Beta-glucosidases (β-glucosidases) are key cellulolytic enzymes that catalyze the hydrolysis of cellobiose to glucose. They are terminal enzymes of the cellulase system as they act during the final step of the cellulose degradation. Beta-glucosidases (β-glucoside glucohydrolases, EC 3.2.1.21; BGL) have been found in the glycoside hydrolase (GH) families GH1, GH3, GH5, GH9, GH30, and GH116 of the CAZy database. They are anomeric configuration-retaining enzymes that operate through the canonical double-displacement glycosidase mechanism, except those of the GH9 family. Here, we report the crystal structure of a β-glucosidase from the thermophilic filamentous fungus Chaetomium thermophilum (CtBGL) at a resolution of 2.99 Å, and compare it with other β-glucosidases of the GH3 family.

The structure of CtBGL consists of three distinct domains, similar to other GH3 family members: A catalytic triose phosphate isomerase (TIM) barrel-like domain (Leu51–Ser354), an α/β sandwich domain (His396–Gly596) and a FnIII (fibronectin type III) domain (Thr663–Gln867) with a prominent insertion region (677–766). A linker region (residues 355–394) connects domain 1 to domain 2 and a second linker region (600–662) connects domain 2 to domain 3. The active site is located in a shallow pocket near the interface of the first and second domain. A molecule of β-d-glucose (BGC) was fitted at the active site based on residual electron density observed in electron density Fo–Fc difference maps. The source of the β-d-glucose is most likely the growth medium used as no β-d-glucose was used during crystallizations or soaking. Two catalytic residues were identified, Asp287 (nucleophile) at the N-terminal TIM-barrel domain and Glu517 (acid/base) at the sandwich α/β domain II. Potential glycosylation sites were observed in the CtBGL structure in 10 positions, all in Asn residues. A total of 27 glycan moieties were found in CtBGL. The N-glycan at CtBGL Asn329 was located in domain I of the enzyme and consisted of eight monosaccharides (two GlcNAc, five α-d-Man, and one β-d-Man). CtBGL has been found to be thermostable at 50 °C and to retain half of its activity after incubation at 65 °C for 55 min.

> WATSEPSYPSPWMNPNAAGWEQAYQWAKDFVSQMTLLEKVNLTTGVGWEGEQCVGQTGAIPRLGLRSLCLHDSPLGIRGTDYNSAFPSGQTTAATWDRTLFYKRGYAMGKEARGKGINVLLGPVAGPLGRMPAGGRNWEGFSPDPVLTGIAMAETVKGIQDAGVIACAKHLIGDEQEHFRQVGDGFDIDESLSSNIDDRTMHELYLWPFADAVRAGVGSVMCAYNQVNNSYSCHNSKLLNGLLKNELGFQGFVMSDWQAQHTGVASAVAGLDMTMPGDTVFNSGLSFWGANLTVAVLNGTLPAYRLDDMAMRIMAAFFKVRGTQDVDLDPINFSFWTLDTYGPIHWGAKEGHQQINFHVDVREDHSRLIREIAAKGTVLLKNEGALPLDKPKFLAVIGEDAGPNHNGPNSCDDRGCVGGTLAMGWGSGTANFPYLVTPDAALQAQAIKDGSRYESVLSNHAMETIRKVVSQDNVTAVVFVNANSGEGYITVDGNRGDRNNLTLWNGGDELIKNVASWCSNTIVVIHSVGPVLLTDWYDHPNITAILWAGLPGQESGNAITDVLYGKVNPAGRSPFTWGATREGYGADVLYDPDDARVPQQNFTEGVFIDYRYFDKHNTRVIYEFGHGLSYTTFEYRNLQIQKHNVSAYIPTTGLTEPAPTFGEHSTNYSDYLYPEGFHRANRYIYPYVNSTDLELASGDPYYGQTADQFLPPNATSSDPQPLLRSSGKNSPGGNPQLYDVLYTVTADITNTGALEGDEVVQLYVSLGGPDDPKVMLRDFARLHIKPGETVKFEGKLTRRDLSTWDVTLQDWVIRDHTKMVFLGKSSRKLVLGALLN>[3x]SMSRITIERDGLTLVGDREEPFGEIYDMAIIMHGFTANRNTDLLRQIADDLRDENVASVRFDFNGHGESDGKFEDMTVCNEIADGKAILDYVHTDPHVRDIFLVG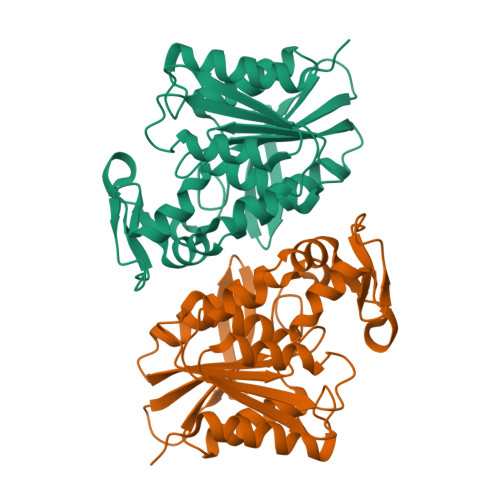HSQGGVVASMLAGLYPDVVKKVVLLAPAAQLKDDALRGNTQGATYDPNHIPDVVPLVGNALGMKVGGFYLRTAQVLPIYEVSQRFTRPVSVIAGTNDQVVDPKYAKKYDEVYENSELHMIPNADHRFSGGYKDMAADLTAQFLKPAF>MLVWLAEHLVKYYSGFNVFSYLPFRAIVSLLTALFISLWMGPRMIAHLQKLSFGQVVRNDGPESHFSKRGTPTMGGIMILTAIVISVLLWAYPSNPYVWCVLVVLVGYGVIGFVDDYRKVVRKDTKGLIARWKYFWMSVIALGVAFALYLAGKDTPATQLVVPFFKDVMPQLGLFYILLAYFVIVGTGNAVNLTDGLDGLAIMPTVFVAGGFALVAWATGNMNFASYLHIPYLR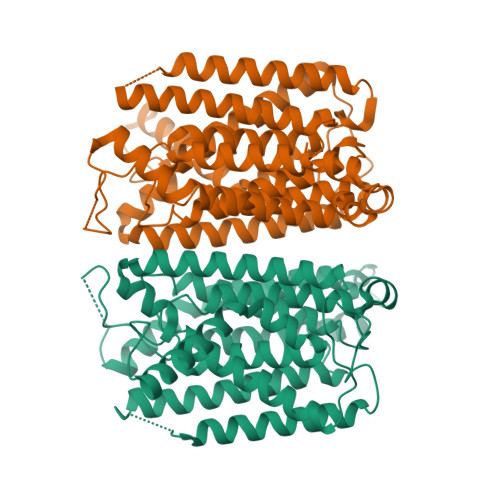HAGELVIVCTAIVGAGLGFLWFNTYPAQVFMGDVGSLALGGALGIIAVLLRQEFLLVIMGGVFVVETLSVILQVGSFKLRGQRIFRMAPIHHHYELKGWPEPRVIVRFWIISLMLVLIGLATLKVR[2x]>PVVDTVHGKVLGKFVSLEGFAQPVAIFLGIPFAKPPLGPLRFTPPQPAEPWSFVKNATSYPPMCTQDPKAGQLLSELFTNRKENIPLKLSEDCLYLNIYTPADLTKKNRLPVMVWIHGGGLMVGAASTYDGLALAAHENVVVVTIQYRLGIWGFFSTGDEHSRGNWGHLDQVAALRWVQDNIASFGGNPGSVTIFGESAGGESVSVLVLSPLAKNLFHRAISESGVALTSVLVKKGDVKPLAEQIAITAGCKTTTSAVMVHCLRQKT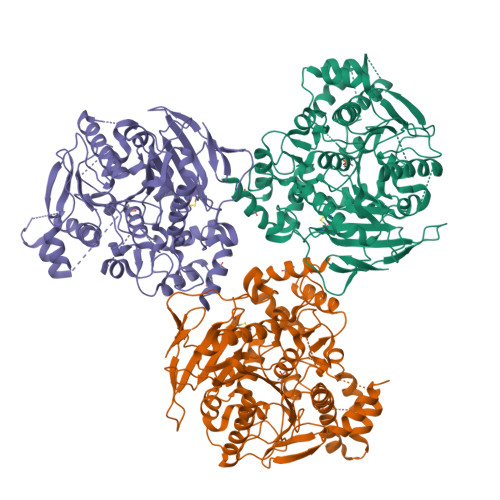EEELLETTLKMKFLSLDLQGDPRESQPLLGTVIDGMLLLKTPEELQAERNFHTVPYMVGINKQEFGWLIPMLMSYPLSEGQLDQKTAMSLLWKSYPLVCIAKELIPEATEKYLGGTDDTVKKKDLFLDLIADVMFGVPSVIVARNHRDAGAPTYMYEFQYRPSFSSDMKPKTVIGDHGDELFSVFGAPFLKEGASEEEIRLSKMVMKFWANFARNGNPNGEGLPHWPEYNQKEGYLQIGANTQAAQKLKDKEVAFWTNLFAK[3x]methyl 2-{[(4-methylpyrimidin-2-yl)carbamoyl]sulfamoyl}benzoate 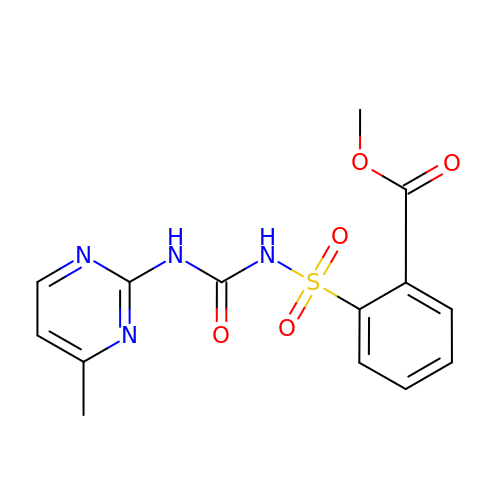| C14 H14 N4 O5 S | VGBNSONMEGTIDX-UHFFFAOYSA-N> GSKKKIDILLKAVGDTPIMKTKK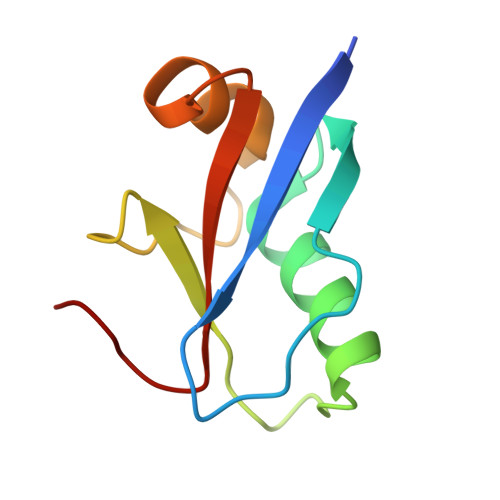WAVERTRTIQGLIDFIKKFLKLVASEQLFIYVNQSFAPSPDQEVGTLYECFGSDGKLVLHYCKSQAWG N~2~-(4-fluorophenyl)-6-{[(5-{[(oxolan-2-yl)methyl]amino}-1,3,4-thiadiazol-2-yl)sulfanyl]methyl}-1,3,5-triazine-2,4-diamine 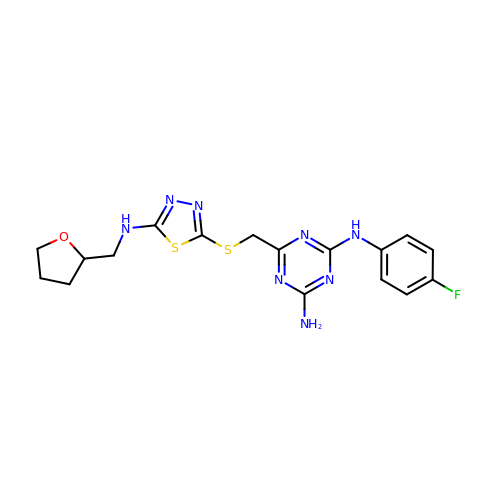| C17 H19 F N8 O S2 | YMCUEXLWILKXTO-UHFFFAOYSA-N> MKKFRKHKRISNCISILLILYLTLGGLLPNNIYAQDLQSYSEKVCNTTYKAPIERPEDFLKDKEKAKEWERKEAERIEQKLERSEKEALESYKKDSVEISKYSQTRNYFYDYQIEANSREKEYKELRNAISKNKIDKPMYVYYFESPEKFAFNKVIRTENQNEISLEKFNEFKETIQNKLFKQDGFKDISLYEPGKGDEKPTPLLMHLKLPRNTGMLPYTNTNNVSTLIEQGYSIKIDKIVRIVIDGKHYIKAEASVVSSLDFKDDVSKGDSWGKANYNDWSNKLTPNELADVNDYMRGGYTAINNYLISNGPVNNPNPELDSKITNIENALKREPIPTNLTVYRRSGPQEFGLTLTSPEYDFNKLENIDAFKSKWEGQALSYPNFISTSIGSVNMSAFAKRKIVLRITIPKGSPGAYLS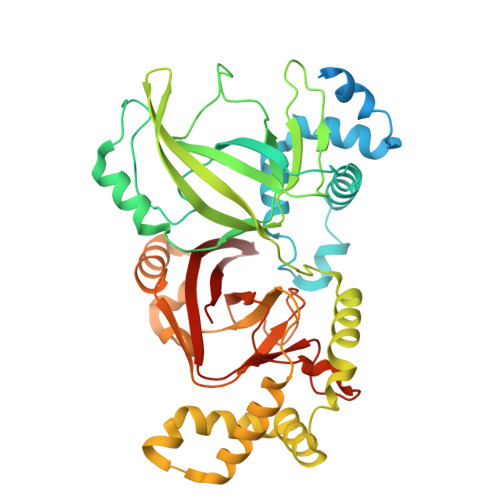AIPGYAGEYEVLLNHGSKFKINKIDSYKDGTITKLIVDATLIP>MSDKDSKNTPQVPEKLGLSRRGFLGASAVTGAAVAATALGGAVMTRESWAQAVKESKQKIHVGPGELDDYYGFWSGGHQGEVRVLGVPSMRELMRIPVFNVDSATGWGLTNESRHIMGDSAKFLNGDCHHPHISMTDGKYDGKYLFINDKANSRVARIRLDIMKCDKMITVPNVQAIHGLRLQKVPHTKYVFANAEFIIPHPNDGKVFDLQDENSYTMYNAIDAETMEMAFQVIVDGNLDNTDADYTGRFAAATCYNSEKAFDLGGMMRNERDWVVVFDIHAVEAAVKAGDFITLGDSKTPVLDGRKKDGKDSKFTRYVPVPKNPHGCNTSSDGKYFIAAGKLSPTCSMIAIDKLPDLFAGKLADPRDVIVGEPELGLGPLHTTFDGRGNAYTTLFIDSQVVKWNMEEAVRAYKGEKVNYIKQKLDVHYQPGHLHASLCETNEADGKWLVALSKFSKDRFLPVGPLHPENDQLIDISGDEMKLVHDGPTFAEPHDCIMARRDQIKTKKIWDRNDPFFAPTVEMAKKDGINLDTDNKVIRDGNKVRVYMTSMAPAFGVQEFTVKQGDEVTVTITNIDQIEDVSHGFVVVNHGVSMEISPQQTSSITFVAD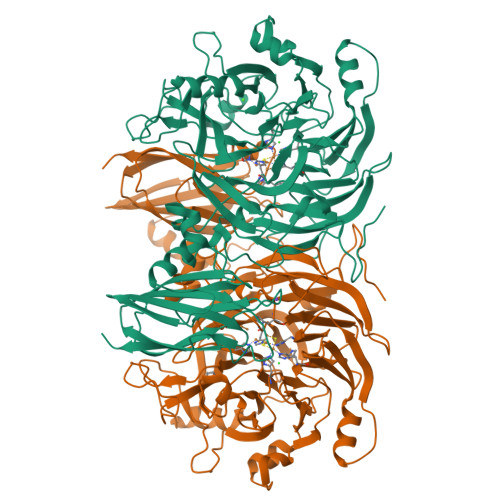KPGLHWYYCSWFCHALHMEMVGRMMVEPA[2x]>[2x]GSADETLSQTKVLLDIFTGVRLYLPPSTPDFSRLRRYFV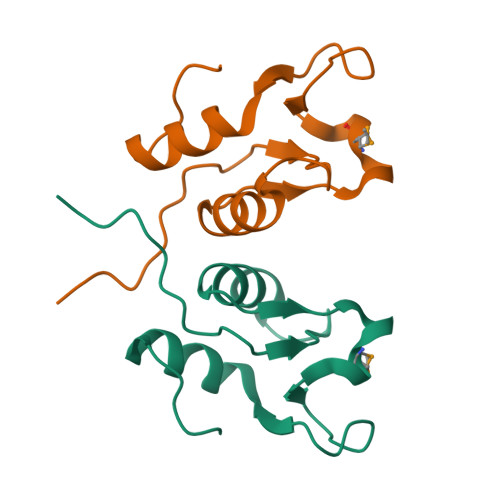AFDGDLVQEFDMTSATHVLGSRDKNPAAQQVSPEWIWACIRKRRLVAPS> QPIFLNVLEAIEPGVVCAGHDNNQPDSFAALLSSLNELGERQLVHVVKWAKALPGFRNLHVDDQMAVIQYSWMGLMVFAMGWRSFTNVNSAMLYFAPDLVFNEYRMHKSRMYSQCVRMRHLSQEFGWLQITPQEFLCMKALLLFSIIPVDGLKNQKFFDELRMNYIKELDRIIACKRK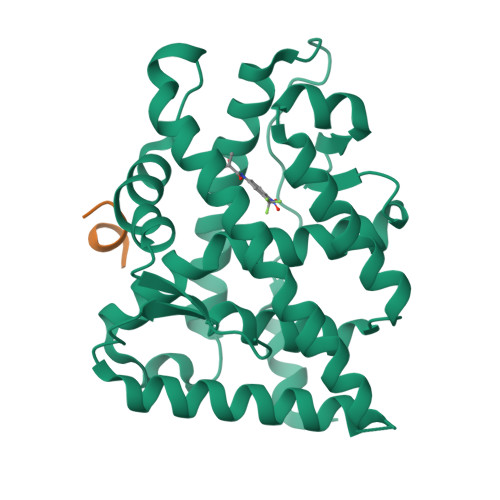NPTSCSRRFYQLTKLLDSVQPIARELHQFAFDLLIKSHMVSVDFPEMMAEIISVQVPKILSGKVKPIYFHTQ;> NTTDTLFSQHYR[(1~{S},2~{S},3~{S},4~{S})-2-(hydroxymethyl)-3,4-bis(oxidanyl)cyclopentyl]azanium | C6 H14 N O3 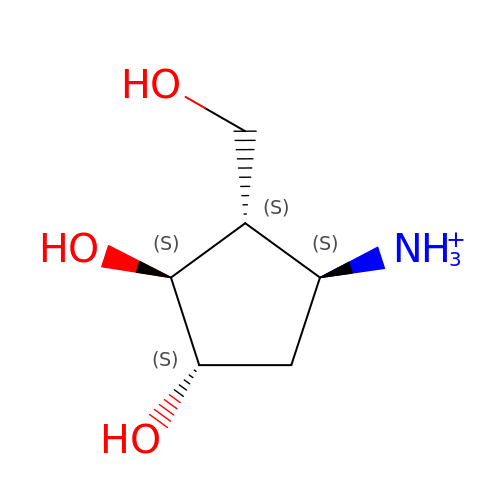| XJKPQBOZNVQXOP-VANKVMQKSA-O>[4x]HGSMTDTYLHETLVFDNKLSYIDNQRDTDG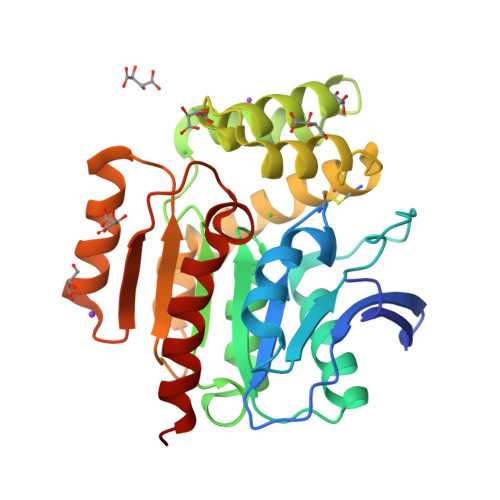PAILLLPGWCHDHRVYKYLIQELDADFRVIVPNWRGHGLSPSEVPDFGYQEQVKDALEILDQLGVETFLPVSHSHGGWVLVELLEQAGPERAPRGIIMDWLMWAPKPDFAKSLTLLKDPERWREGTHGLFDVWLDGHDEKRVRHHLLEEMADYGYDCWGRSGRVIEDAYGRNGSPMQMMANLTKTRPIRHIFSQPTEPEYEKINSDFAEQHPWFSYAKLGGPTHFPAIDVPDRAAVHIREFATAIRQGQ>GSSHHHHHHSSGENLYFQHMASWDIFCSVVDNYGDIGVTWRLARQLAAEHGQAVRLWVDEPQAFARICPRADPVAHVQCLDGVEVRAWGRPWAPVAAADVVIEAFACELPEAHRQAMRERKRPSLWLNLEYLSAEEWIGSCHALPSLQACGLSKYFFFPGFREPSGGLLREAGLLERRRRFQASVSAQDEFLASLGVRRKVGERLISLFAYENPALPGWLEQLRDARQPSLLLVPEGRVLADVADWLRVATLAVGDVHVRDALRVQVLPFMAQDDYDRLLWCCDLNAVRGEDSFVRAQWAGRPLLWHIYRQEEETHLAKLEAFLELYCAGLPADLAENLRTFWLAWNAGGGLAGAWEGLERQLPEWRREAQRWADEQGMRPDLAARLVQFYADWL[2x];>GSSHHHHHHSSGENLYFQHMKTAQEFRAGQVANINGAPWVIQKAEFNKSGRNAAVVKMKLKNLLTGAGTETVFKADDKLEPIILDRKEVTYSYFADPLYVFMDSEFNQYEIEKDDLEGVLTFIEDGMTDICEAVFYNDKVISVELPT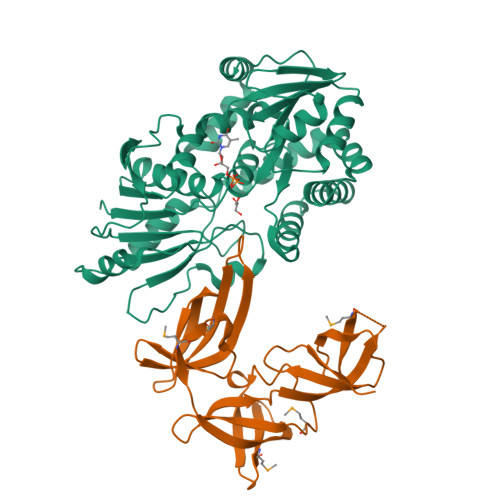TIVRQIAYTEPAVRGDTSGKVMKTARLNNGAELQVSAFCEIGDSIEIDTRTGEYKSRVKA[2x]>MDPYSETSDLVDISRFDTHGLGANYKLRRHKFEHLADTGCHKARSDWVKYIGPLTEFGGCNHINGNFSAV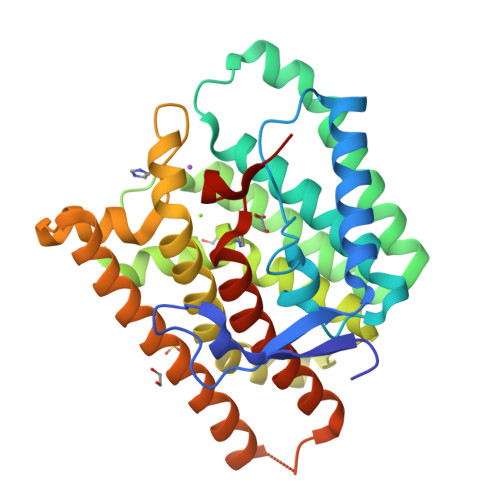VLPLCRPDRLELIAYVLEFAFLHDSVLESENTSPESEVQAEAGLRLLYERCISRLLQTDEVCAKKIAKTWKDAINTTTKDKNVDFQSIEDYLEFRMIDTGAPFVEALMLFGLGMSLSPQEDDALGHVIRPCFAALALTNDYFSFDREIEEVDTSTLINSVAIVMRIQSLDIPTAKTIINETIQKYEREFLRRIDEYKQHKGPISNKIEQYMEAMTYQISGNLVWSLNCPRYNPDYRYGLEACQHEG[2x]2-(6-oxidanyl-3-oxidanylidene-cyclohexa-1,4-dien-1-yl)ethanoic 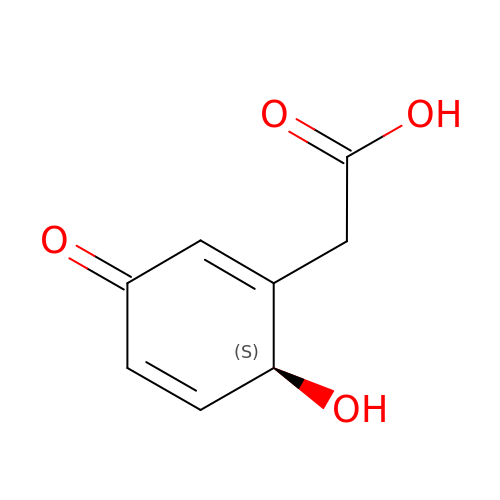acid | C8 H8 O4 | SORMFPBLGIOKJT-ZETCQYMHSA-N>AKQFTKCELSQLLKDIDGYGGIALPELICTMFHTSGYDTQAIVENNESTEYGLFQISNKLWCKSSQVPQSRNICDISCDKFLDDDITDDIMCAKKILDIKGIDYWLAHKALCTEKLEQWLCEKL[2x];> ASMTGGQQMGRGSASLPACPEESPLLVGPMLIEFNMPVDLELVAKQNPNVKMGGRYAPRDCVSPHKVAIIIPFRNRQEHLKYWLYYLHPVLQRQQLDYGIYVINQAGDTIFNRAKLLNVGFQEALKDYDYTCFVFSDVDLIPMNDHNAYRCFSQPRHISVAMDKFGFSLPYVQYFGGVSALSKQQFLTI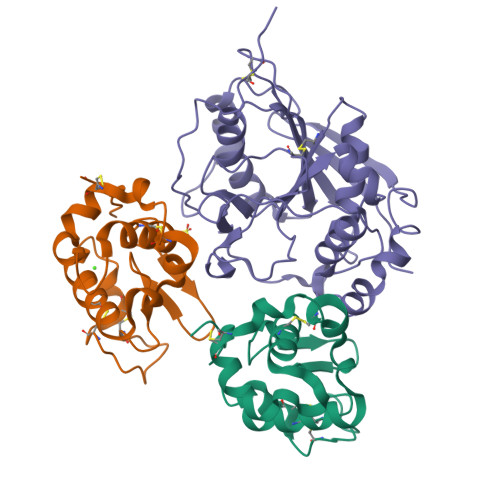NGFPNNYWGWGGEDDDIFNRLVFRGMSISRPNAVVGTTRMIRHSRDKKNEPNPQRFDRIAHTKETMLSDGLNSLTYQVLDVQRYPLYTQITVDIGTPS>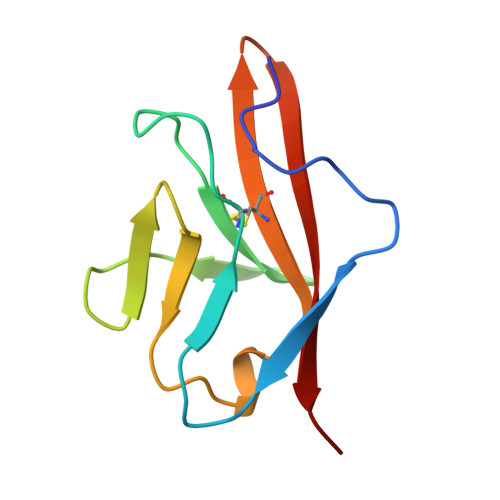 GRPFVEMYSEIPEIIHMTEGRELVIPCRVTSPNITVTLKKFPLDTLIPDGKRIIWDSRKGFIISNATYKEIGLLTCEATVNGHLYKTNYLTHRQT>[2x]MAEIGTGFPFDPHYVEVLGERMHYVDVGPRDGTPVLFLHGNPTSSYVWRNIIPHVAPTHRCIAPDLIGMGKSDKPDLGYFFDDHVRFMDAFIEALGLEEVVLVIHDWGSALGFHWAKRNPERVKGIAFMEFIRPIPTWDEWPEFARETFQAFRTTDVGRKLIIDQNVFIEGTLPMGVVRPLTEVEMDHYREPFLNPVDREPLWRFPNELPIAGEPANIVALVEEYMDWLHQSPVPK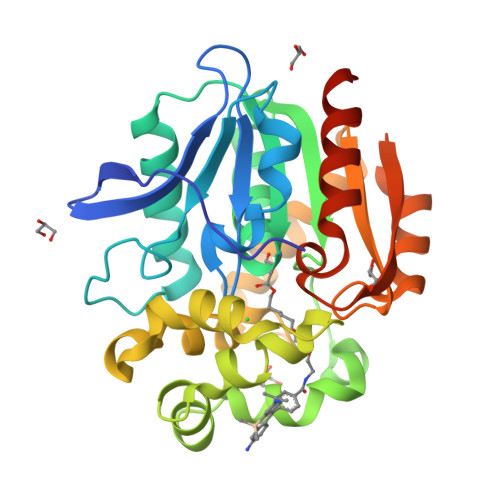LLFWGTPGVLIPPAEAARLAKSLPNCKAVDIGPGLNLLQEDNPDLIGSEIARWLSTLEISGHHHHHH> MGSSHHHHHHHSSGRENLYFQGHMEGVRWAFSCGTWLPSRAEWLLAVRSIQPEEKERIGQFVFARDAKAAMAGRLMIRKLVAEKLNIPWNHIRLQRTAKGKPVLAKDSSNPYPNFN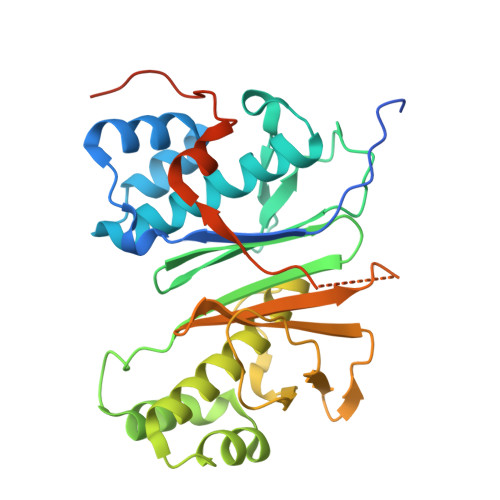FNISHQGDYAVLAAEPELQVGIDIMKTSFPGRGSIPEFFHIMKRKFTNKEWETIRSFKDEWTQLDMFYRNWALKESFIKAIGVGLGFELQRLEFDLSPLNLDIGQVYKETRLFLDGEEEKEWAFEESKIDEHHFVAVALRKPDGSRHQDVPSQDDSKPTQRQFTILNFNDLMSSAVPMTPEDPSFWDCFCFTEEIPIRNGTKS>MAFRATLSFAGKEFDVLDCTYSLKRDVDSKGRPSSNIYGGQIRLHVESTDDTSILENMTNQFKPHSGSIVFKKGDEEAKMKELTWENGYITEFTENIDIVGSQPMTITFVVSAQVIKIGGAQFEQNWPK[6x];>[3x]MASTNLDAVSVEIKVAGKVCDYVTMELFQSVSTHHRFKIKVNYRPDKPSVWAIGPDVIFKQLGEKVSIIMTHHESGEKTEFHGLISDIHVEGFDGNQGFVILEGGSPTILLDRDPAMDCYVEQNLNTIVSDILDKSGVKMNVTNNPKHTDIIPYVARYKETSYGFLSRLLRSYGEWFYYNGETLQIGDPEIDTESRAGYDVDLTGVSINATIRSLNHSTYEFDPVNDKFYYDYSGTPKGATLGSRSAEKCSEPIFPTEAKLPSIRPAYSAMDLEHYGDAGFHRNYSQLSQIKASSRYCGIRLGELVVTRVPESFPGVKITDLGRYRITEITHTVNYKGQYSNTFCGVPGGTPIMPWGDAVMPVAYPEMARVVSNDDPKNQGRVKVQFMWQEVDGGESYWMRVQSPDAGKSEQVAKNRGFVFIPEPGDLVMVGFEQGNPDRPYVTGSLFYKANSEGAATDNTVKSMRTRSGHTLEFKDDEGGDWGITLRDINGNVIHLNSKDKNIDITAPETITLTAKNVCINTEENVQITAKKNIDMTVEADINSSAKGNLLLQADKDVLTAAKGNVGIEAKSDINMVGKNIAVEGN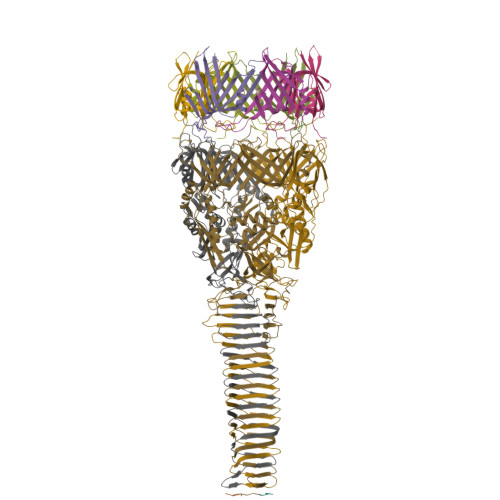SKITLNGGQTQVAGQQTTIQGAANKIEIM;>[3x]MKQIVTINLNHICPMVTGVTPHIGGPIIGPGCPGVMVNGVPISVMGDMCVCCGPPDTIVQGEPGILVNGKPIVLQGCMTAHGGIIPAGVPGVTVSSASPIEPITMNHVSPKRNRFLAAISGNNLQEAIENQNALQKKMLEEEPMIFNVHWEKEDIHIAESHINKKVTVNADTIGFKDGETVKFVITPEAIDTANGEQVEDIELTGTVNNNHVTVEWIVELKK[2-(2-hydroxyethoxy)ethoxy]acetic acid | C6 H12 O5 | 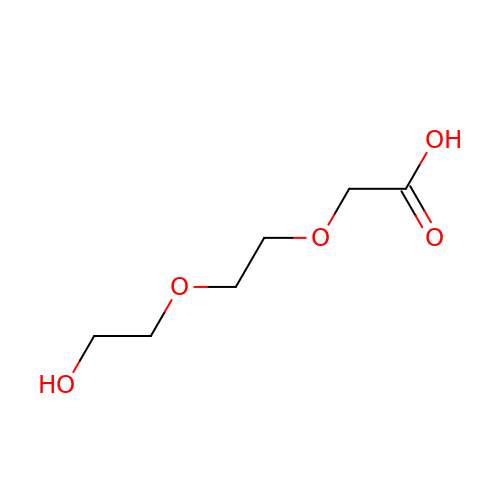PRBXPAHXMGDVNQ-UHFFFAOYSA-N>[10x]GKFSRALKN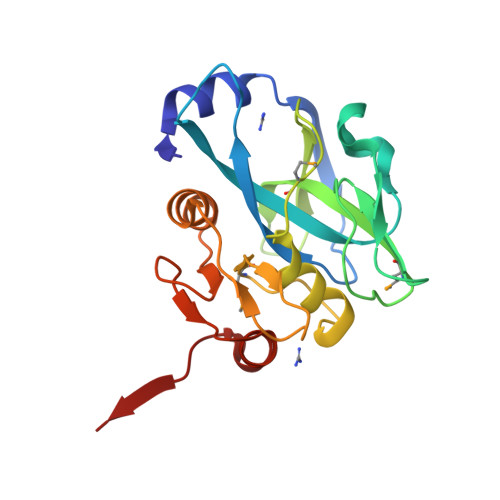RLESANYEEVELPPPSKGVIVPVVHTVKSAPGEAFGSLAIIIPGEYPELLDANQQVLSHFANDTGSVWGIGEDIPFEGDNMCYTALPLKEIKRNGNIVVEKIFAGPIMGPSAQLGLSLLVNDIEDGVPRMVFTGEIADDEETIIPICGVDIAAIAAHEQGLPLIGNQPGVDEEVRNTSLAAHLIQTGTLPVQRA> MRGSFANDATFEIKKCDLHRLEEGPPVTTVLTREDGLKYYRMMQTVRRMELKADQLYKQKIIRGFCHLCDGQEACCVGLEAGINPTDHLITAYRAHGFTFTRGLSVREILAELTGRKGGCAKGKGGSMHMYAKNFYGGNGIVGAQVPLGAGIALACKYNGKDEVCLTLYGDGAANQGQIFEAYNMAALWKLPCIFICENNRYGMGTSVERAAASTDYYKRGDFIPGLRVDGMDILCVREATRFAAAYCRSGKGPILMELQTYRYHGHSMSDPGVSYRTREEIQEVRSKSDPIMLLKDRMVNSNLASVEELKEIDVEVRKEIEDAAQFATA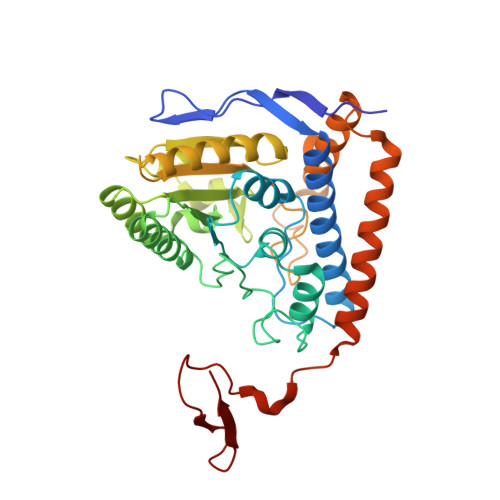DPEPPLEELGYHIYSSDPPFEVRGANQWIKFKSVS>[2x]KDDMKAAEQYQGAASAVDPAHVVRTNGAPDMSESEFNEAKQIYFQRCAGCHGVLRKGATGKPLTPDITQQRGQQYLEALITYGTPLGMPNWGSSGELSKEQITLMAKYIQHTPPQPPEWGMPEMRESWKVLVKPEDRPKKQLNDLDLPNLFSVTLRDAGQIALVDGDSKKIVKVIDTGYAVHISRMSASGRYLLVIGRDARIDMIDLWAKEPTKVAEIKIGIEARSVESSKFKGYEDRYTIAGAYWPPQFAIMDGETLEPKQIVSTRGMTVDTQTYHPEPRVAAIIASHEHPEFIVNVKETGKVLLVNYKDIDNLTVTSIGAAPFLHDGGWDSSHRYFMTAANNSNKVAVIDSKDRRLSALVDVGKTPHPGRGANFVHPKYGPVWSTSHLGDGSISLIGTDPKNHPQYAWKKVAELQGQGGGSLFIKTHPKSSHLYVDTTFNPDARISQSVAVFDLKNLDAKYQVLPIAEWADLGEGAKRVVQPEYNKRGDEVWFSVWNGKNDSSALVVVDDKTLKLKAVVKDPRLITPTGKFNVYNTQHDVY

Denitrification is the stepwise reduction of nitrogen oxides to dinitrogen and is utilized by many bacteria to replace the terminal oxygen-dependent steps of the respiratory chain under anaerobic conditions. The reduction of nitrite to nitric oxide is a highly regulated step, since both of these molecules are toxic to the cell. In NirS, these domains form homodimers by interaction of the 15th β-strand of each subunit, which is consistent with the SEC data collected during purification (data not shown). 1 nitrite reductase NirS adopts an open and a closed conformation, and it has been hypothesized that these states are linked to the catalytic cycle.

1 are likely to be caused by inherent properties of the cofactor.> PELPEVETIRRTLLPLIVGKTIEDVRIFWPNIIRHPRDSEAFAARMIGQTVRGLERRGKFLKFLLDRDALISHLRMEGRYAVASALEPLEPHTHVVFCFTDGSELRYRDVRKFGTMHVYAK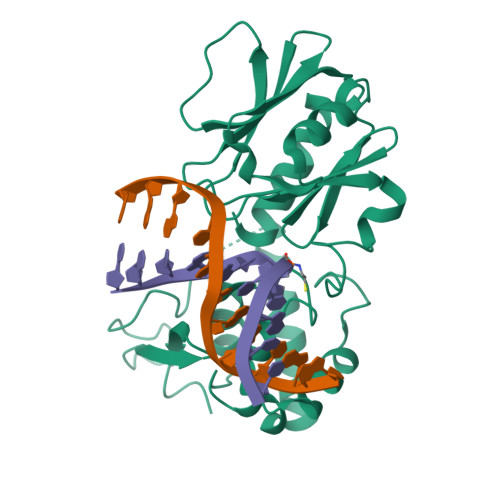EEADRRPPLAELGPEPLSPAFSPAVLAERAVKTKRSVKALLLDCTVVAGFGNIYVDESLFRAGILPGRPAASLSSKEIERLHEEMVATIGEAVMKGGSTPRTYVNTQGEAGTFQHHLYVYGRQGNPCKRCGTPIEKTVVAGRGTHYCPRCQR N-acetyl-beta-neuraminic 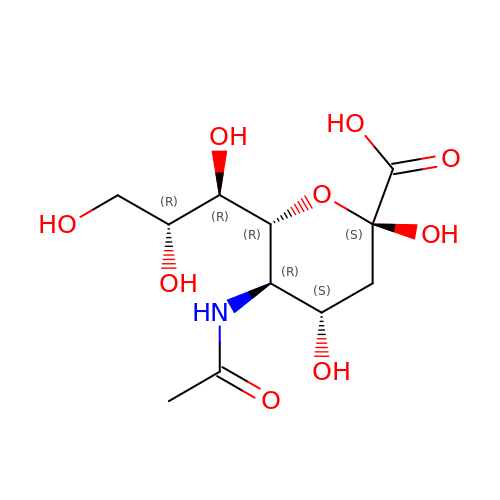acid | C11 H19 N O9 | SQVRNKJHWKZAKO-PFQGKNLYSA-N>SNAMLHYVHVGNKKSPNTLLFVHGSGCNLKIFGELEKYLEDYNCILLDLKGHGESKGQCPSTVYGYIDNVANFITNSEVTKHQKNITLIGYSMGGAIVLGVALKKLPNVRKVVSLSGGARFDKLDKDFMEKIYHNQLDNNYLLECIGGIDNPLSEKYFETLEKDPDIMINDLIACKLIDLVDNLKNIDIPVKAIVAKDELLTLVEYSEIIKKEVENSELKIFETGKHFL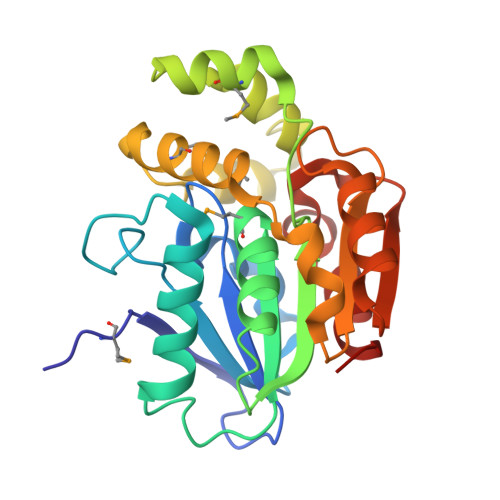LVVNAKGVAEEIKNFI[2x]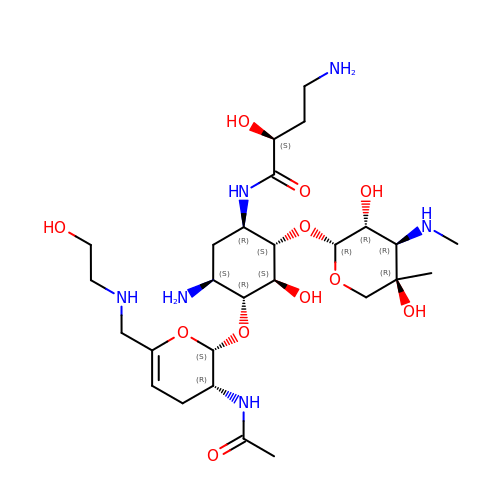(2S)-N-[(1R,2S,3S,4R,5S)-4-{[(2S,3R)-3-(acetylamino)-6-{[(2-hydroxyethyl)amino]methyl}-3,4-dihydro-2H-pyran-2-yl]oxy}-5-amino-2-{[3-deoxy-4-C-methyl-3-(methylamino)-beta-L-arabinopyranosyl]oxy}-3-hydroxycyclohexyl]-4-amino-2-hydroxybutanamide | C27 H50 N6 O11 | PALSFHNAOHBRHX-ARRQPEMVSA-N Mitogen-activated protein kinase kinase kinase kinase 1 (MAP4K1) is a serine/threonine kinase that acts as an immune checkpoint downstream of T-cell receptor stimulation. MAP4K1 activity is enhanced by prostaglandin E2 (PGE2) and transforming growth factor beta (TGFβ), immune modulators commonly present in the tumor microenvironment. Therefore, its pharmacological inhibition is an attractive immuno-oncology concept for inducing therapeutic T-cell responses in cancer patients. Through its proline-rich domain, MAP4K1 binds to a diversity of adaptors in hematopoietic cells, including those involved in T-cell receptor (TCR), B-cell receptor, and cytokine-induced signaling. The function of MAP4K1 has been studied most extensively in the context of T-cell activation.

Encouraged by the properties of 11, we synthesized fluorine containing oxetane 12, which showed a comparable activity and selectivity profile, accompanied by reduced in vivo clearance (CLb = 1.3 L/h/kg) and improved bioavailability (F = 69%). However, the overall kinase selectivity of this molecule, in addition to its stability profile, revealed significant challenges. Not only did 12 show instability under basic conditions due to the known lability of trifluoromethyl groups at the C3 position of azaindoles, but the oxazine moiety also displayed rapid degradation under acidic conditions. In addition to challenges with hydrolytic stability, 12 also displayed plasma instability. Most problematic though were cardiovascular toxicities driven by residual ROCK2 activity that were observed in an in vivo rat telemetry study, where 12 produced a dose-dependent decrease in mean arterial blood pressure (MAP) after a single dose (10, 15, 30% reduction compared to baseline in MAP at 15, 30, and 60 mg/kg of 12 respectively). Furthermore, 12 showed a positive signal in the micronucleus test, a result which we attributed to the overall unfavorable kinase selectivity displayed by 12, in addition to the lack of Rho kinase selectivity. With these parameters in mind, a further campaign was initiated with the goal of improving both the stability and the kinase selectivity profile of 12.

>DIFNRDPRDHYDLLQRLGGGTYGEVFKARDKVSGDLVALKMVKMEPDDDVSTLQKEILILKTCRHANIVAYHGSYLWLQKLWICMEFCGAGSLQDIYQVTGSLSELQISYVCREVLQGLAYLHSQKKIHRDIKGANILINDAGEVRLADFGISAQIGATLARRLSFIGTPYWMAPEVAAVALKGGYNELCDIWSLGITAIELAELQPPLFDVHPLRVLFLMTKSGYQPPRLKEKGKWSAAFHNFIKVTLTKSPKKRPSATKMLSHQLVSQPGLNRGLILDLLDKLKNP[2x]>[2x]MLTFALTIVRHGETQYNRDKLLQGQGIDTPLSDTGHQQAAAAGRYLKDLHFTNVFVSNLQRAIQTAEIILGNNLHSSATEMILDPLLRERGFGVAEGRPKEHLKNMANAAGQSCRDYTPPGGETLEQVKTRFKMFLKSLFQRMFEEHGSALSSVPSEADQPVIAGLADDGAQNVPVHALMVSHGAFIRISVRHLVEDLQ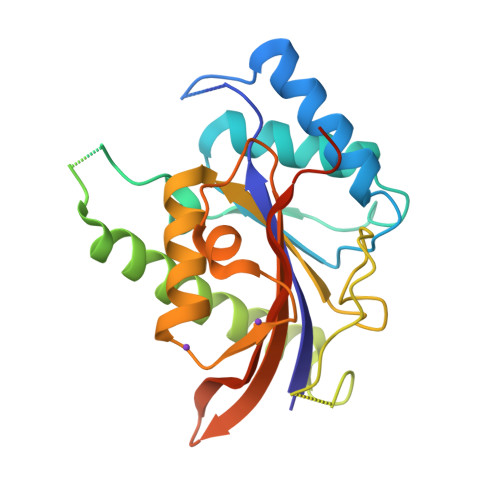CCLPAGLKMNQVFSPCPNTGISRFIFTIHREESVLRATRIQGVFINRKDHLEEVKNSDLEHHHHHH> MFLQDLIFMISEEGAVAYDPAANECYCASLSSQVPKNHVSLVTKENQVFVAGGLFYNEDNKEDPMSAYFLQFDHLDSEWLGMP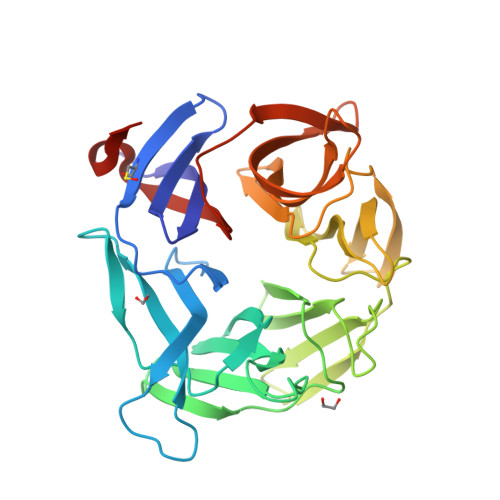PLPSPRCLFGLGEALNSIYVVGGREIKDGERCLDSVMCYDRLSFKWGESDPLPYVVYGHTVLSHMDLVYVIGGKGSDRKCLNKMCVYDPKKFEWKELAPMQTARSLFGATVHDGRIIVAAGVTDTGLTSSAEVYSITDNKWAPFEAFPQERSSLSLVSLVGTLYAIGGFATLETESGELVPTELNDIWRYNEEEKKWEGVLREIAYAAGATFLPVRLNVLRLTKMAENLYFQ In this study, we identify a family of complement inhibitors from the hard tick Rhipicephalus pulchellus, hereafter termed CirpA (Complement inhibitor from R. pulchellus of the alternative pathway). Functional and structural characterisation reveals that members of the CirpA family directly bind to properdin, inhibiting its ability to promote complement activation, and leading to potent inhibition of the complement response in a species specific manner. Whilst many molecules act to control inappropriate activation, Properdin is the only known positive regulator of the human complement system. All CirpA structures share a lipocalin fold with a short N-terminal α-helix followed by an eight-stranded beta-barrel and a longer C-terminal α-helix.

Using this strategy, we were able to purify CirpA1, A3, A4, and A5 and determine their structure using X-ray crystallography to a resolution of 2.0, 2.1, 1.8, and 1.9 Å respectively. Overall, the structures appear very similar, with the biggest conformational differences in the tilt angle of the C-terminal helix H2 as well as variations in loops between beta strands 4 and 5 (L4-5) and between strands 7 and 8 (L7-8). We identified three regions with high conformational variability between homologs. All these regions are part of the observed binding interface between CirpA1 and properdin, and hence the conformational differences might render other homologs incompatible with binding human properdin. Another CirpA1 residue undergoing a conformational rearrangement upon properdin binding is Y122 which forms a hydrophobic pocket around properdin P377 together with CirpA1 residues F122, Y131, and F150. This pocket is incomplete in all three CirpA1 homolog structures. However, it is likely that the homologues have evolved to target properdin from other species, especially given the identification of multiple CirpA homologues in a single tick species.

> MGNEQDSEIYRFDQFMNTDDYIWVFNTTQEGPKECEKDKKHNMTNDKIIFVRSHQEETKIVNETIIGDFFHYSDNKSVYDGIYISGDKREVHAEHLYYSSEDMICGLVQVFARQTDAWTELRVRGRRSYKSLDEVCRTQYEKYVEAIKHTKTSTSPYRDDCQ> MRFVNTLPLIFGLTAALGSSMALALPSDREQPIRVQADSAELDDKQGVAVYRGDVVVTQGSTKLTGNTVTLKQDKNGDIEVVTSVGKPAYYEQKPAPDKD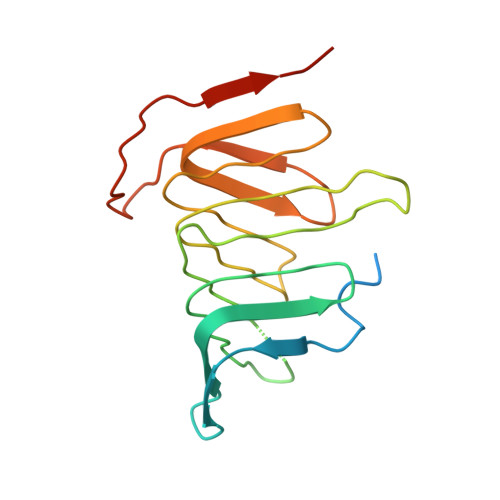VTKAYGLTIQYFVTQNRVVLIDQAKVIQEGNTFEGEKIVYDTQRQIVNAGRATGSQVTSPRPRIDMVIQPKKKAQ ALLOSAMIZOLINE 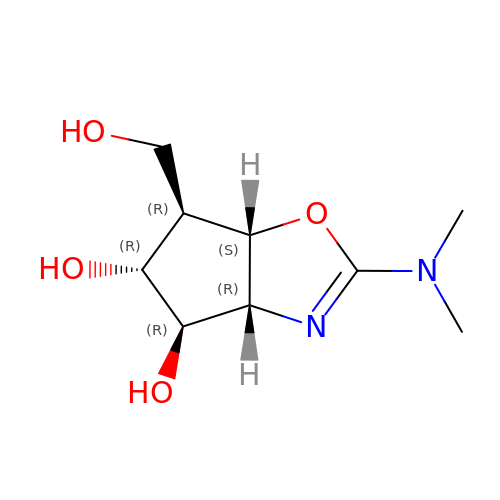| C9 H16 N2 O4 | MKJAYSJDHSEFRI-PVFLNQBWSA-N>MNPAAEAEFNILLATDSYKVTHYKQYPPNTSKVYSYFECREKKTENSKLRKVKYEETVFYGLQYILNKYLKGKVVTKEKIQEAKDVYKEHFQDDVFNEKGWNYILEKYDGHLPIEIKAVPEGFVIPRGNVLFTVENTDPECYWLTNWIETILVQSWYPITVATNSREQKKILAKYLLETSGNLDGLEYKLHDFGYRGVSSQETAGIGASAHLVNFKGTDTVAGLALIKKYYGTKDPVPGYSVPAAEHSTITAWGKDHEKDAFEHIVTQFSSVPVSVVSDSYDIYNACEKIWGEDLRHLIVSRSTQAPLIIRPDSGNPLDTVLKVLEILGKKFPVTENSKGYKLLPPYLRVIQGDGVDINTLQEIVEGMKQKMWSIENIAFGSGGGLLQKLTRDLLNCSFKCSYVVTNGLGINVFKDPVADPNKRSKKGRLSLHRTPAGNFVTLEEGKGDLEEYGQDLLHTVFKNGKVTKSYSFDEIRKN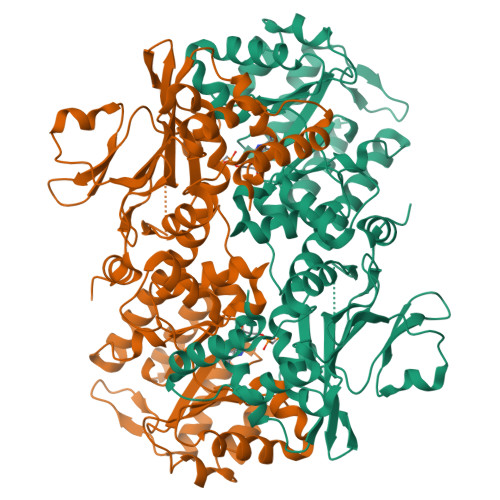AQLNI[2x]> GHMAKTDRSQPSVLARIAAFRTGLSAEASAADYLERQGYRILARRFKTRCGEIDLVAQRDALVAFVEVKARGNVDDAAYAVTPRQQSRIVAAAEAWLSRHPEHAMSELRFDAILIAPNTAPRHLPGAFDA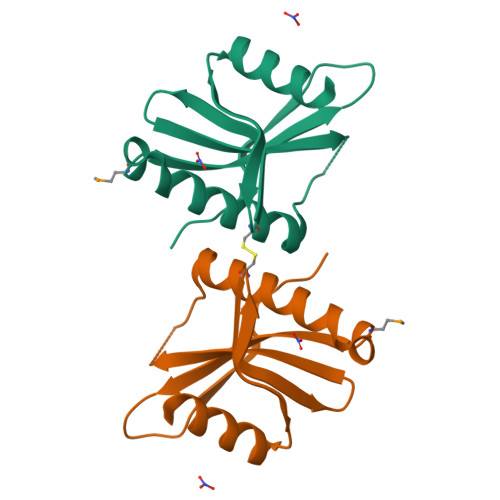TPGS> MAPYGADTPTACCFSY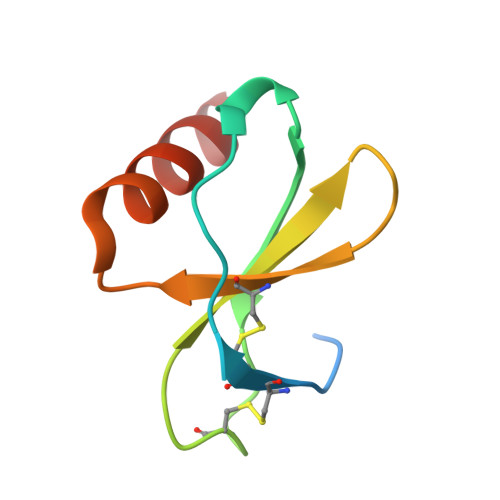SRKIPRQFIVAYFETSSLCSQPGVIFLTKRNRQICADSKETWVQEYITDLELNA>[10x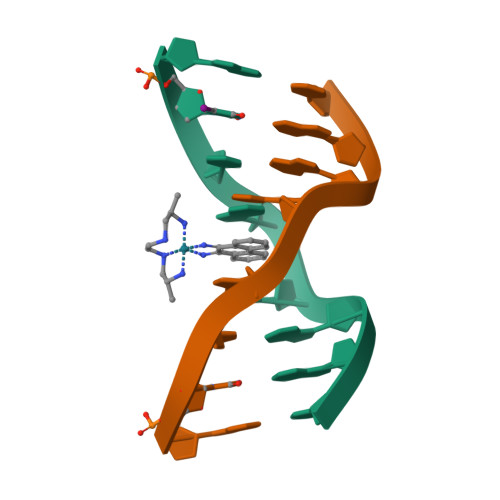]GUTGCAAC>XTYSITLRVFQRNPGRGFFSIVEKTVFHYANGGTWSEAKGTHTLTMGGSGTSGVLRFMSDKGELITVAVGVHNYKRWCDVVTGLKPEETALVINPQYYNNGPRAYTREKQLAEYNVTSVVGTRFEVKYTVVEGNNLEANVIFS[4x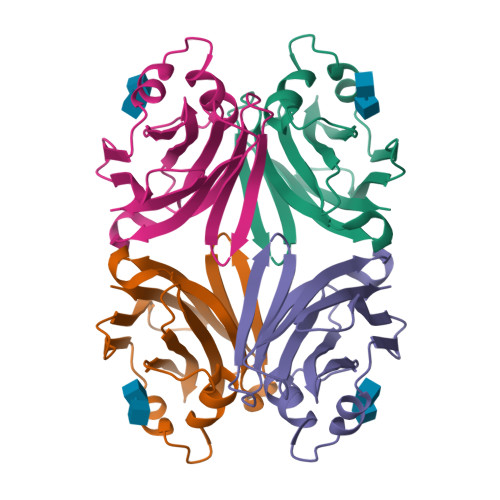]> MISAKTLRPAIAAIALFAIGATG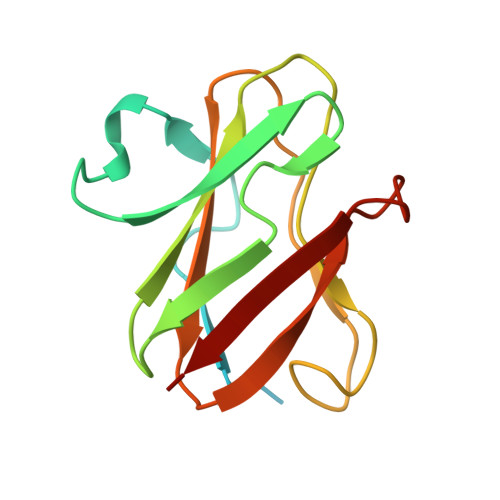AWAQDKITVTSEKPVAAADVPADAVVVGIEKMKYLTPEVTIKAGETVYWVNGEVMPHNVAFKKGIVGEDAFRGEMMTKDQAYAITFNEAGSYDYFCTPHPFMRGKVIVE> KPKGHPHMNSIRIDGDITLGGLFPVHGRGSEGKPCGELKKEKGIHRLEAMLFALDRINNDPDLLPNITLGARILDTCSRDTHALEQSLTFVQALIEKDGTEVRCGSGGPPIITKPERVVGVIGASGSSVSIMVANILRLFKIPQISY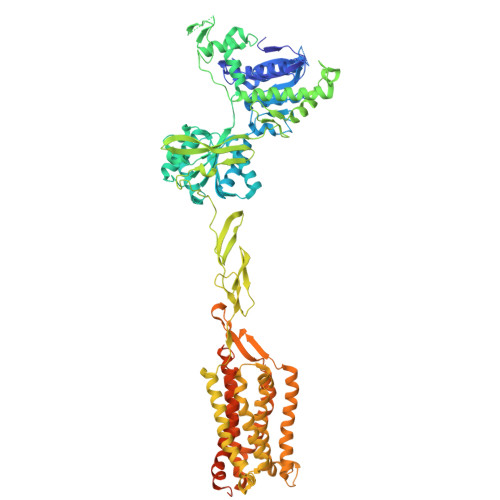ASTAPDLSDNSRYDFFSRVVPSDTYQAQAMVDIVRALKWNYVSTVASEGSYGESGVEAFIQKSREDGGVCIAQSVKIPREPKAGEFDKIIRRLLETSNARAVIIFANEDDIRRVLEAARRANQTGHFFWMGSDSWGSKIAPVLHLEEVAEGAVTILPKRMSVRGFDRYFSSRTLDNNRRNIWFAEFWEDNFHCKLSRHALKKGSHVKKCTNRERIGQDSAYEQEGKVQFVIDAVYAMGHALHAMHRDLCPGRVGLCPRMDPVDGTQLLKYIRNVNFSGIAGNPVTFNENGDAPGRYDIYQYQLRNDSAEYKVIGSWTDHLHLRIERMHWPGSGQQLPRSICSLPCQPGERKKTVKGMPCCWHCEPCTGYQYQVDRYTCKTCPYDMRPTENRTGCRPIPIIKLEWGSPWAVLPLFLAVVGIAATLFVVITFVRYNDTPIVKASGRELSYVLLAGIFLCYATTFLMIAEPDLGTCSLRRIFLGLGMSISYAALLTKTNRIYRIFEQGKRSVSAPRFISPASQLAITFSLISLQLLGICVWFVVDPSHSVVDFQDQRTLDPRFARGVLKCDISDLSLICLLGYSMLLMVTCTVYAIKTRGVPETFNEAKPIGFTMYTTCIVWLAFIPIFFGTSQSADKLYIQTTTLTVSVSLSASVSLGMLYMPKVYIILFHPEQNVPKRKRSLKAVVTAATMSNKFTQKGNFRPNGEAKSELCENLEAPALATKQTYVTYTNHAI> MGSSHHHHHHSSGLVPAGSHAGMIIAADYITEDGKPIIRIFKKEKGEFKVEYDRTFRPYIYALLKDDSAIDEVKKITAERHGKIVRITEVEKVQKKFLGRPIEVWKLYLEHPQDVPAIREKIREHPAVVDIFEYDIPFAKRYLIDKGLTPMEGNEELTFLAVDIETLYHEGEEFGKGPIIMISYADEEGAKVITWKSIDLPYVEVVSSEREMIKRLVKVIREKDPDVIITYNGDNFAFPYLLKRAEKLGIKLPLGRDNSEPKMQRMGDSLAVAI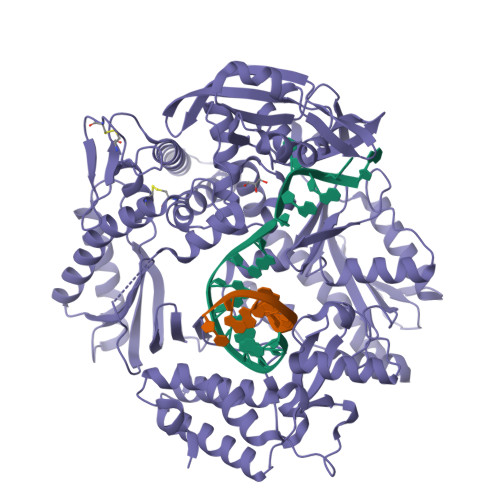KGRIHFDLFPVIRRTINLPTYTLEAVYEAIFGKSKEKVYAHEIAEAWETGKGLERVAKYSMEDAKVTFELGKEFFPMEAQLARLVGQPVWAVSRSSTGNLVEWFLLRKAYERNELAPNKPDEREYERRLRESYEGGYVKEPEKGLWEGIVSLDFRSLYPSIIITHNVSPDTLNRENCKEYDVAPQVGHRFCKDFPGFIPSLLGNLLEERQKIKKRMKESKDPVEKKLLDYRQRAIKILANSYYGYYGYAKARWYCKECAESVTAWGRQYIDLVRRELESRGFKVLYIDTDGLYATIPGAKHEEIKEKALKFVEYINSKLPGLLELEYEGFYARGFFVTKKKYALIDEEGKIVTRGLEIVRRDWSEIAKETQAKVLEAILKHGNVDEAVKIVKEVTEKLSKYEIPPEKLVIYEQITRPLSEYKAIGPHVAVAKRLAAKGVKVKPGMVIGYIVLRGDGPISKRAIAIEEFDPKKHKYDAEYYIENQVLPAVERILRAFGYRKEDLKYQKTKQVGLGAWLKF> MTLGDLWKRRLNNCTKEEFFAYRRTGILETERDKARELLRKGETNMGLAVSRGTAKLAWLEERGYVNLKGEVVDLGCGRGGWSYYAASRPAVMGVKAYT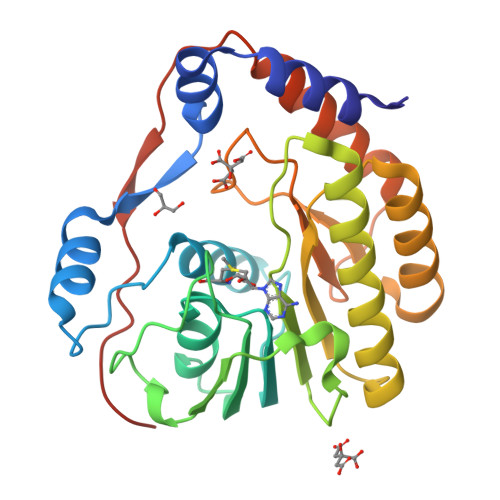IGGKGHEAPKMVTSLGWNLIKFRAGMDVFTMQPHRADTVMCDIGESSPDAAIEGERTRKVILLMEQWKNRNPSASCVFKVLAPYRPEVIEALHRFQLQWGGGLVRTPFSRNSTHEMYYSTAISGNIVNSVNVQSRKLLARFGDQRGPIRVPEMDLGVGTRHHHHHH>[4x]GSRMSGNNMSTPLPAIVPAARKATAAVIFLHGLGDTGHGWAEAFAGIRSSHIKYICPHAPVRPVTLNMNVAMPSWFDIIGLSPDSQEDESGIKQAAEN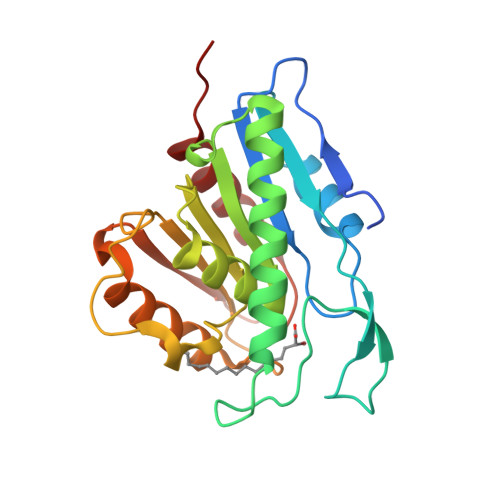IKALIDQEVKNGIPSNRIILGGFSQGGALSLYTALTTQQKLAGVTALSCWLPLRASFPQGPIGGANRDISILQCHGDCDPLVPLMFGSLTVEKLKTLVNPANVTFKTYEGMMHSSCQQEMMDVKQFIDKLLPPID> ELKVVTATNFLGTLEQLAGQFAKQTGHAVVISSGSSGPVYAQIVNGAPYNVFFSADEKSPEKLDNQGFALPGSRFTYAIGKLVLWSAKPGLVDNQGKVLAGNGWRHIAISNPQIAPYGLAGTQVLTHLGLLDKLTAQERIVEANSVGQAHSQTASGAADLGFVALAQIIQAAAKIPGSHW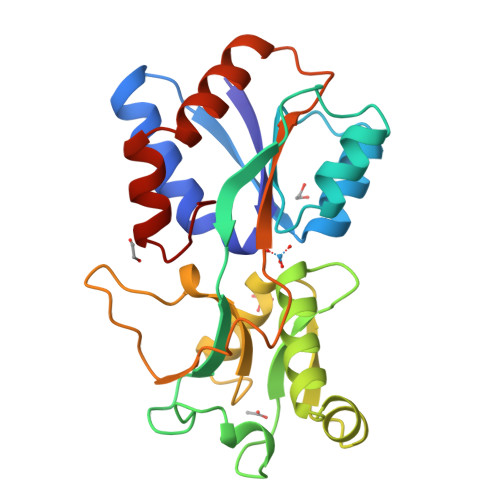FPPANYYEPIVQQAVITKSTAEKANAEQFMSWMKGPKAVAIIKAAGYVLPQ>[4x]MKVEEILEKALELVIPDEEEVRKGREAEEELRRRLDELGVEYVFVGSYARNTWLKGSLEIDVFLLFPEEFSKEELRERGLEIGKAVLDSYEIRYAEHPYVHGVVKGVE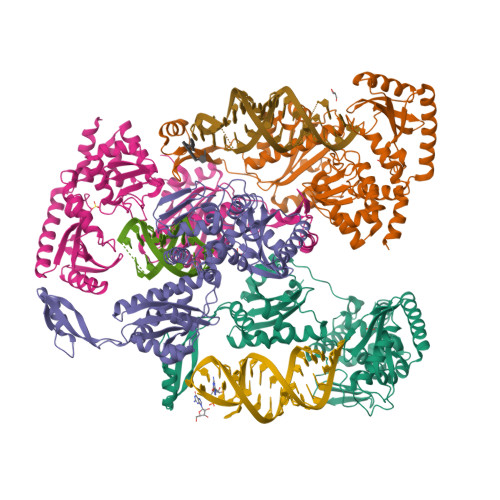VDVVPCYKLKEPKNIKSAVDRTPFHHKWLEGRIKGKENEVRLLKGFLKANGIYGAEYKVRGFSGYLCELLIVFYGSFLETVKNARRWTRRTVIDVAKGEVRKGEEFFVVDPVDEKRNVAANLSLDNLARFVHLCREFMEAPSLGFFKPKHPLEIEPERLRKIVEERGTAVFAVKFRKPDIVDDNLYPQLERASRKIFEFLERENFMPLRSAFKASEEFCYLLFECQIKEISRVFRRMGPQFEDERNVKKFLSRNRAFRPFIENGRWWAFEMRKFTTPEEGVRSYASTHWHTLGKNVGESIREYFEIISGEKLFKEPVTAELCEMMGVKDSNSSSVDKLAAALEHHHHHH Two glycosyltransferases (GTases), SdgB and SdgA, are responsible for the glycosylation of S. aureus SDR proteins such as ClfA and ClfB. SdgB first appends N-acetyl­glucosamine (GlcNAc) moieties onto serine residues (O-glycosylation) within the SDR domain using uridine diphos­phate N-acetylglucosamine (UDP-GlcNAc) as a donor substrate. The subsequent addition of GlcNAc to the glycoproteins is catalyzed by the second enzyme, SdgA, yielding glycosylated SDR proteins in which each SD repeat is decorated with GlcNAc disaccharide moieties. The glycosylation of SDR proteins mediated by SdgA and SdgB protects SDR proteins from degradation by host proteases, thereby circumventing innate immune attack.

Despite the biological significance of these two glycosyltransferases involved in pathogenicity and avoidance of the host innate immune response, their structures and the molecular basis of their activity have not been investigated. This study reports the crystal structures of SdgB and SdgA from S. aureus as well as multiple structures of SdgB in complex with its substrates (for example UDP, N-acetylglucosamine or SDR peptides), products (glycosylated SDR peptides) or phosphate ions. Altogether, the extensive snapshots of SdgB complexes in multiple states provided a mechanistic insight into how SdgB recognizes and glycosylates the clustered serine residues in the SDR proteins.

>MNYFVGNSLGVNLTGIEKAIINRLNLFKEMGRPAQCVFLSWNRYLYRNAQNYITSSDYINMYDFFQEATYLERNEPFDWLSYWTDECHYTLKHVENSHDFRIYDQERFLMYAHFQDPKYRILDYVNHFDSQRRKVKRDFYDVRGFLSCSRILVDKQQTLCEFFYNPEGDTKLEKYFSYKDGKPEVQKIIVYYANKQYFFNNETELGAFFIKQLYQHGDLFFSDRNVYTAPIFNLTPESIPVVAVLHSTHIKNIDALDSSPFKNVYKAMFENLSRYRAIIVSTEQQKLDVEKRINHTIPVVNIPVGYSETIDTPVQTLDQRSVKLISVARYSPEKQLHQQIELIKRLVSYVPKIELHMYGFGSESKKLNELIQKYGLENHVYLRGFLSNLDQEYSDAYLSLITSNMEGFSLALLESLAHGVPVISYDIKYGPNELITSDFNGYLITKNDEDALFDKVKYVIDHPEVQQRLSKGSLAKAQQYSKASLIKQWDQFVRLILEHHHHHH[2x]N-{4-[(2-amino-4-oxo-4,7-dihydro-3H-pyrrolo[2,3-d]pyrimidin-5-yl)methyl]benzene-1-carbonyl}-D-glutamic acid | C19 H19 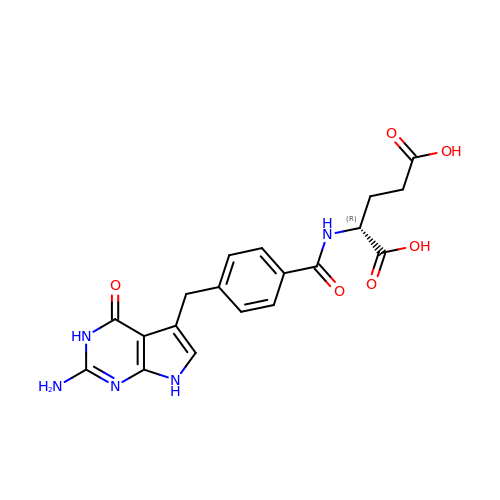N5 O6 | VDHBMZRBPMTLGE-GFCCVEGCSA-N>[2x]ACPAPPPGQPDIRAIGYYTDKAGSVIDPALQQQNKDATAPLDRYAADVARMSDDYLRNGDPAAAQCTLSWLGAWADDGAMLGQMIRVNNDQSFYMRQWMLDAVAMAYLKVHDQANPQQRARIDPWLQKLARANLAYW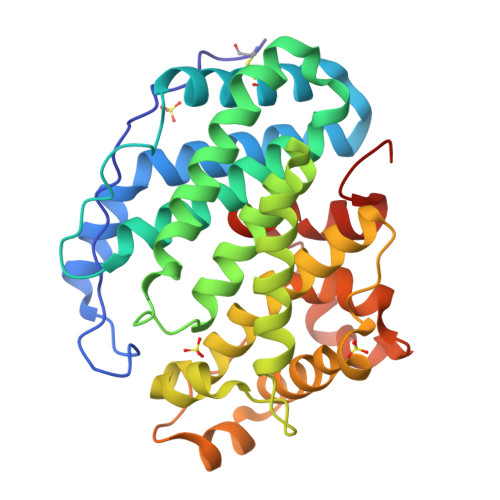DNPKRRRNNHYYWGGLGVLATGLATDDDALWQAGHAAFQKGIDDIQDDGSLPLEMARGQRALHYHDYALAPLVMMAELARLRGQDWYASRNHAIDRLARRVIEGSRDPAWFNQHTGAAQLPLQASGWVEFYRLRSPDGGVFDAAHARGPFHSPRLGGDLTLMATHGIVRTPLRHHHHHH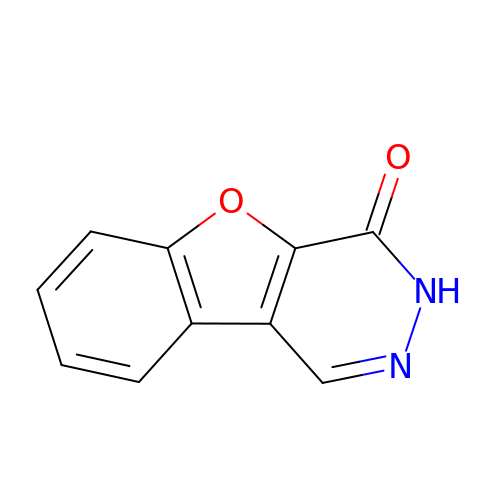[1]benzofuro[2,3-d]pyridazin-4(3H)-one | C10 H6 N2 O2 | JPYPDSHHTRFKAI-UHFFFAOYSA-N> SSSIFQLRLQEFANERGMLANGRPCEPGCRTFFRICLKHYQATFSEGPCTFGNVSTPVLGTNSFVIRDKNSGSGRNPLQLPLNFTWPGTFSLNIQAWHTPGDDLRPETSPGNSLISQIIIQGSLAVGKNWKSDEQNNTLTRLRYSYRVVCSDNYYGDSCSRLCKKRDDHFGHYECQPDGSPSCLPGWTGKYCDQPICLSGCHEQNGYCSKPDECNCRPGWQGPLCNECIPHKGCRHGTCTIPWQCACDEGWG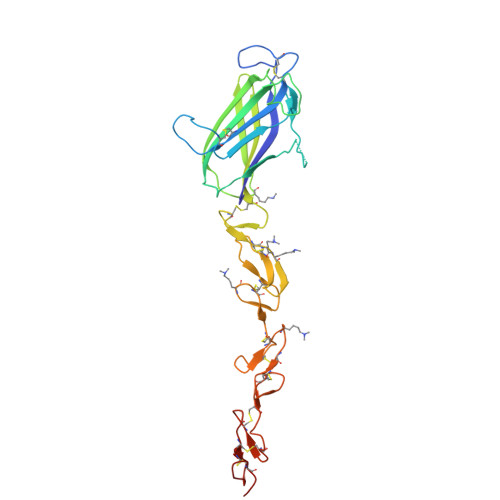GLFCDQAAA In addition to their membrane‐bound chlorophyll a/c light‐harvesting antenna, the cryptophyte algae have evolved a unique phycobiliprotein antenna system located in the thylakoid lumen. The basic unit of this antenna consists of two copies of an αβ protomer where the α and β subunits scaffold different combinations of a limited number of linear tetrapyrrole chromophores. While the β subunit is highly conserved, encoded by a single plastid gene, the nuclear‐encoded α subunits have evolved diversified multigene families. By careful examination of three newly determined crystal structures in comparison with three previously obtained, we show how the α subunit amino acid sequences control chromophore conformations and hence spectral properties even when the chromophores are identical.

The crystal structure of PC630 from Chroomonas gentoftensis CCAC1627 was determined at 1.8 Å resolution. The structure shows a closed form cryptophyte PBP. This protein is very similar to the previously examined PC645 from “Chroomonas” sp. CCMP270 (RMSD 0.324 Å over 2732 atoms). Although the chemical structures of all the chromophores are identical between PC645 and PC630, a careful examination of structural details showed that the key difference between them was a twist along the bond between pyrrole ring D and ring C in the PCB attached to β82. In PC630, Gln6 in both αL and αS makes a side chain hydrogen bond to the nitrogen atom in pyrrole ring D of the β82 chromophore. In contrast, Gln6 of PC630 is replaced by Leu5 in each α subunit of PC645. Leu5 sterically prevents pyrrole ring D of chromophore β82 adopting the same orientation as all other cryptophyte structures. Thus, the sequence of the α subunit N‐terminal segment dictates the twist of pyrrole ring D of the β82 phycocyanobilin (PCB) chromophore and hence the spectral difference between PC630 and PC645. The α19 chromophore on PC630 αL shows a very slight bowing between pyrrole rings B and C, which is not present in any of the other α19 chromophores in PC630 or PC645. This is likely to be due to sequence differences in the chromophore loop of PC630 αL that result in the disruption of a conserved salt bridge that stabilizes the conformation of the α chromophore (see Section 2.8).

> AIKKDQKAPIITIFDNRGCEVKKNNYSGAKANGMEDDQCVKLTMETITVSETTAAKKLQEFIGLKATAINVPQISGVTKKY;>FSRVVTNADSKAAYVGGADLQALKKFVSEGNKRLDAVNAIVSNASCIVSDAVSGMICENPALISPSGNCYTNRRMAACLRDAEIILRYVSYSLLSGDSSVLEDRCLSGLKETYSSLGVPTAGNLRAVGIMKATCVAFINNTSQQKKLSTPAGDCSALASEVAGYFDKVSAALA[2x];> AIKKDQKAPVVTIFDARGCKDHSNKEYTGAKAGGMEDDQCVKLTMETIKVGDDVAAKVLGECLSELKSRK> IVGGTNSSWGEWPWQVSLQVKLTAQRHLCGGSLIGHQWVLTAAHCFDGLPLQDVW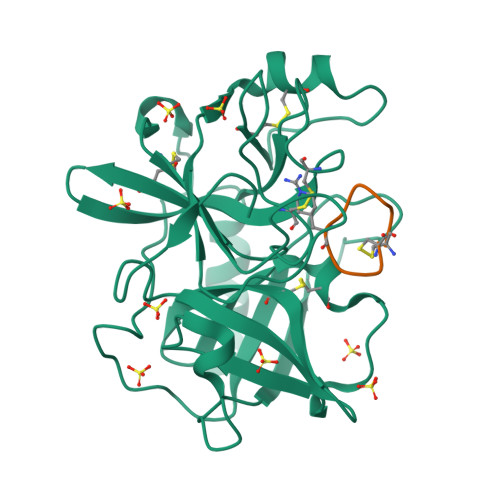RIYSGILNLSDITKDTPFSQIKEIIIHQNYKVSEGNHDIALIKLQAPLNYTEFQKPISLPSKGDTSTIYTNCWVTGWGFSKEKGEIQNILQKVNIPLVTNEECQKRYQDYKITQRMVCAGYKEGGKDACKGDSGGPLVCKHNGMWRLVGITSWGEGCARREQPGVYTKVAEYMDWILEKTQSSD;> CPARFAALWC> GRRASVELNEKPLPEGWEMRFTVDGIPYFVDHNRRTTTYIDPRTGK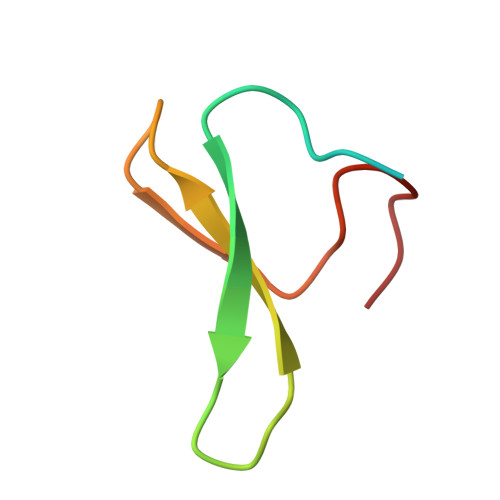S> MQTVNEMLRRAATRAPDHCALAVPARGLRLTHAELRARVEAVAARLHADGLRPQQRVAVVAPNSADVVIAILALHRLGAVPALLNPRLKSAELAELIKRGEMTAAVIAVGRQVADAIFQSGSGARIIFLGDLVRDGEPYSYGPPIEDPQREPAQPAFIFYTSGTTGLPKAAIIPQRAAESRVLFMSTQVGLRHGRHNVVLGLMPLYHVVGFFAVLVAALALDGTYVVVEEFRPVDALQLVQQEQVTSLFATPTHLDALAAAAAHAGSSLKLDSLRHVTFAGATMPDAVLETVHQHLPGEKVNAYGTTE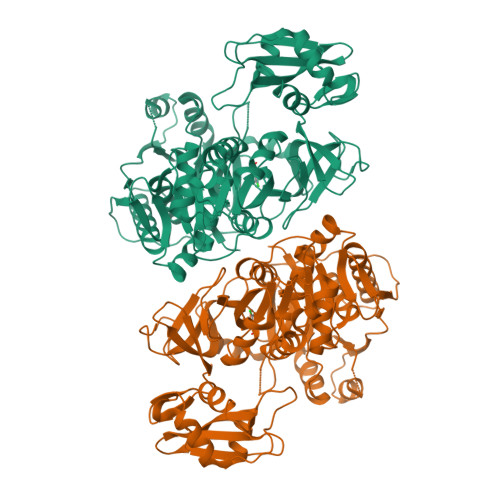AMNSLYMRQPKTGTEMAPGFFSEVRIVRIGGGVDEIVANGEEGELIVAASDSAFVGYLNQPQATAEKLQDGWYRTSDVAVWTPEGTVRILGRVDDMIISGGENIHPSEIERVLGTAPGVTEVVVIGLADQRWGQSVTACVVPRLGETLSADALDTFCRSSELADFKRPKRYFILDQLPKNALNKVLRRQLVQQVSS>SQSTRKKSRRNKWHFGVRCRGDAPEILLAVYRALQRAGAQFTVPK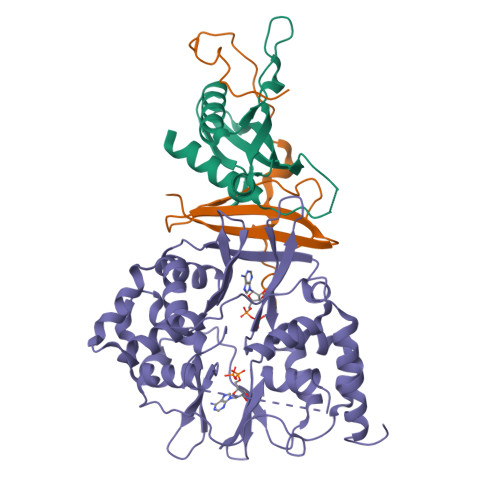PVNGKYRSDMYTIKSRWEIPHCKREGKNTYAYIELQLYEVMPGCFMLDVKSNGYKDIYSHPERTADHGMDDLKSSFPFLDLCAMLVCKLFSA[2x];>MSESEQYSTEIPAFLTSNTLQELKLPKPPSLPPHLEKCILNSNTAYKEDQSVLPNPNHVLLNHLAAANTQLGVLALSATTRYHRKYVTTAMFKNFDV[2x];>AMDVQETQKGALKEIQAFIRSRTSYDVLPTSFRLIVFDVTLFVKTSLSLLTLNNIVSAPLWDSEANKFAGLLTMADFVNVIKYYYQSSSFPEAIAEIDKFRLLGLREVERKIGAIPPETIYVHPMHSLMDACLAMSKSRARRIPLIDVDGETGSEMIVSVLTQYRILKFISMNCKETAMLRVPLNQMTIGTWSNLATASMETKVYDVIKMLAEKNISAVPIVNSEGTLLNVYESVDVMHLIQDGDYSNLDLSVGEALLKRPANFDGVHTCRATDRLDGIFDAIKHSRVHRLFVVDENLKLEGILSLADILNYIIYDKTTTPGVPEQTDNFESAV[2x]> MPEVVFGSVTDLGYAAGWRLVRAMPEAMAQGVFGAGARYAARNGGPEQLRRNLARVVGKPPADVPDDLIRASLASYARYWREAFRLPAMDHGRLGEQLDVIDIDHLWSALDAGRGAVLALPHSGNWDMAGVWLVQNYGPFTTVAERLKPESLYRRFVEYRESLGFEVLPLTGGERPPFEVLAERLTDNRPICLMAERDLTRSGVQVDFFGEATRMPAGPAKLAIETGAALFPVHCWFEGDGWGMRVYP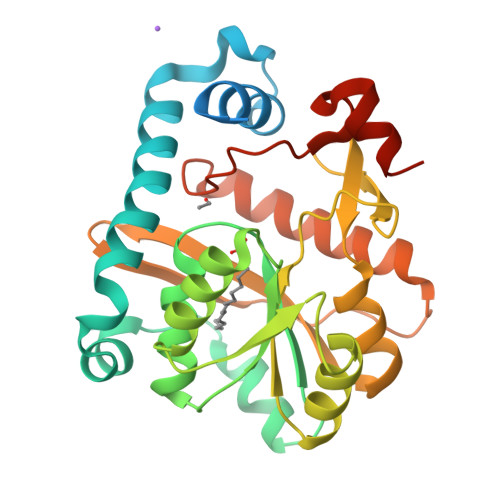ELDTSSGDVTAITQALADRFAANIATYPADWHMLQPQWIADLSDERRARLGTSRHHHHHH> MTSSPVTPSAVDDAPDWPAAFVRRYLDAGHWQDQSFAEALATSAARHPRRIALCDDDQRLSYADLLQRCRRLAAGLRQAGLAHGDTVVLHLPNGIAFVETCFALFQLGVRPVLALPAHRQHEISGFCRFAEAKAYIGAERIDGFDPRPMARELLASGACRMALIHGEAEAPLQALA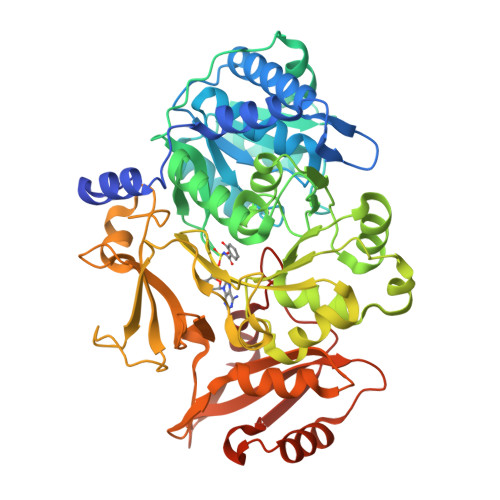PLYQADALEDCAARAEDIACFQLSGGTTGTPKLIPRRHREYLYNVRASAEVCGFDEHTVYLTGLPMAHNFTLCCPGVIGTLLASGRVVVSQRADPEHCFALIARERVTHTALVPPLAMLWLDAQESRRADLSSLRLLQVGGSRLGSSAAQRVEPVLGCQLQQVLGMAEGLICYTRLDDPPERVLHTQGRPLSPDDEVRVVDAEGREVGPGEVGELTVRGPYTIRGYYRLPEHNAKAFSADGFYRTGDRVSRDKDGYLVVEGRDKDQINRGGEKIAAEEVENLLIAHPQVHDATVVAMPDSLLGERTCAFVIPRQPAPSALKLKQYLHACGLAAFKVPDRIELVPAFPQTGIGKISKKDLRERLRRELEARA> MSVLPGAAAIAGIGATEFSKNSGRSELQLACEAVLAAIADAGLEPSDVDGLVTFTADTSSEIHVARNTGIGELKFFSRVGYGGGAACGTVQQAAMAVATGIAEVVVCYRAFNERSGVRYGLGQAGRQMDQGADSAAYAWLLPFGLNTPAQWVAMFARRYMHEYGATSEDFGRVAVVDRKHAATNPKAWFYQRPITLEDHQNSRWIVEPLHLLDCCQES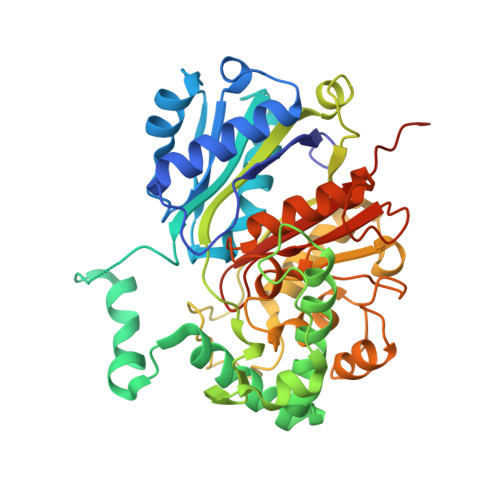DGGQALVVVSTERARDLPHPPALIWGAAQGSGYDQHMMTSYYRSEITGIPEMGLVGQQLYAQSGLNPSDIGAAILYDHFTPLVLPQLEELGFCARGEAKDFIADGNLEIGGRLPCNTHGGQLGEAYIHGMNGIAEAVRLVRGTSVNQPGDVTNVLVTAGTGVPTSGLILGADRKLRSLEHHHHHH> NAPVFTQPEYHISVKENLPVGTRLLTIKATDPDEGVNGEVTYSFRNVREKISQLFQLNSLTGDITVLGELDYEDSGFYDVDVEAHDGPGLRARSKVLVTVLDVNDNAPEVTVTSLTSSIQEASSPGTVIALFNVHDSDSGENGLVTCSIPDNLPFRLEKTYGNYHRLLIHRTLDREEVSDYNITITATDQGTPPLSTETYISLQVVDINDNPPTFTHASYSAYIPENNPRGASILSITAQDPDSGENAQVIYSLSEDTIQGAPMSSYVSINSNTGVLYALRSFDYEQFQDLKLLVTARDSGTPPLSSNVSLSLS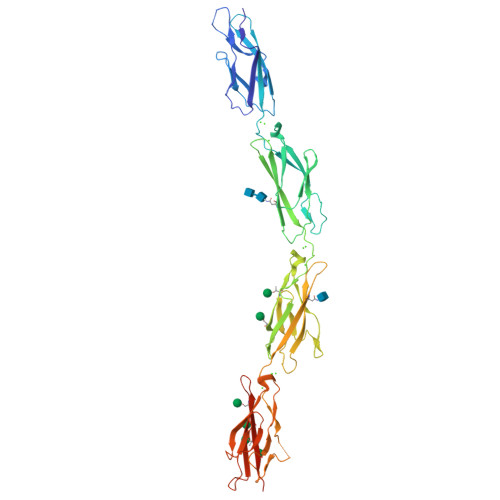VLDQNDNTPEILYPTIPTDGSTGVELTPRSADPGYLVTKVVAVDKDSGQNAWLSYRLLKASEPGLFSVGLHTGEVRTARALLDRDALKQSLVVTVQDHGQPPLSATVTLTIAVSDNIPDHHHHHHHH> KVLLDIFTGVRLYLPPSTPDF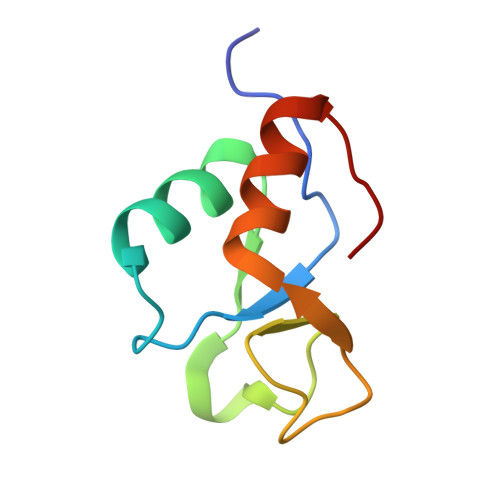SRLRRYFVAFDGDLVQEFDMTSATHVLGSRDKNPAAQQVSPEWIWACIRKRRLVAPS>[12x]GSMELRVGNKYRLGRKIGSGSFGDIYLGANIASGEEVAIKLECVKTKHPQLHIESKFYKMMQGGVGIPSIKWCGAEGDYNVMVMELLGPSLEDLFNFCSRKFSLKTVLLLADQMISRIEYIHSKNFIHRDVKPDNFLMGLGKKGNLVYIIDFGLAKKYRDARTHQHIPYRENKNLTGTARYASINTHLGIEQSRRDDLE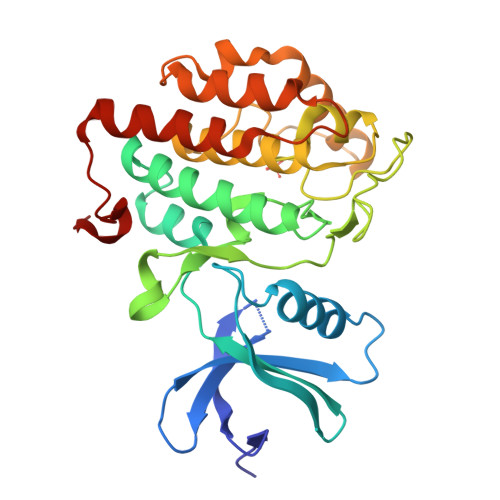SLGYVLMYFNLGSLPWQGLKAATKRQKYERISEKKMSTPIEVLCKGYPSEFSTYLNFCRSLRFDDKPDYSYLRQLFRNLFHRQGFSYDYVFDWNMLK>MHEQYQAPLPVNSPALPEPFYYLHNFRAVLAWIGERYADLLDDQERAFIAAFAELPEASQALLVRMVMRKGTLFREGKLAYAEIGDTRAAVQPLLALGWVDAQPTLELAQLFGLLKKDELSQLFRDHLGRANLRKDALLERLQPLFPEARRLAEWQADFA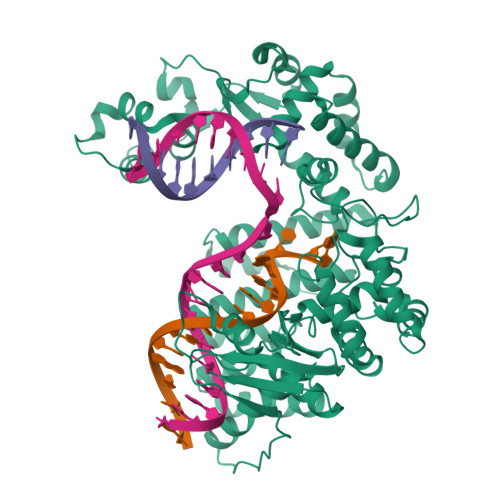EPVYELRCMALCDRLRLMYFGNLWQDWSEFVLADLGIYRYESVEFSADSRGFRLRADVDAYLHLFDCRQRFDLGEPLEELLAGLPGEPYANPWLEGRRVKLLFQFAQHCEKQRDFDLAQRLYRQSSHPGARLRAIRSLERGERFAEAHALAREASCAPESDAERQGLARLLPRLQGKLGLPRQARAAAPEIDRLDLCLAFPSEPCSVEWAVREHLEEPGCAVHYVENGLINSLFGLLCWEAIFAAIPGAFFHPFHSAPADLHSADFRQRRAALFEACLGRLEDGSYRDAIRCRYRDKFGLQSPFVYWELLGEELLEQALDCLPAAHLRAWFERLLEDIPGNRAGLPDLIQFWPAQRRYRMVEVKGPGDRLQDNQLRWLQFCREREMPVAVCYVRWHVDD[2x]Although highly effective vaccines exist for EV71, no vaccine is available for the global public health threats imposed by CVA6, which underscores the critical need for developing an effective vaccine. Here, we demonstrate the isolation of two stable CVA6 particles with excellent natural antigenicity: one empty (CVA6 procapsid) and the other infectious (CVA6 A-particle). The capsid structures of CVA6 procapsid and A-particle at near atomic (~3 Å) resolution both closely resemble those of the uncoating intermediates of other enteroviruses. The cryoEM structures of the CVA6 procapsid, A-particle, and A-particle-1D5 immune-complex we report here reveal atomic resolution details about molecular determinants in CVA6 related to virus neutralization, cell binding, and RNA release.

The top band exhibited a λ260/λ280 absorbance ratio of 0.71, and the particles in that band sedimented with a coefficient of 84S, had a capsid protein composition consistent with the presence of VP0, VP1, and VP3 in sodium dodecyl supfate–polyacrylamide gel electrophoresis (SDS–PAGE) gel electrophoresis (lane 2), and showed an absence of packaged genome as verified by negative stain electron microscopy. These characteristics are all consistent with this band being composed of purified procasids. A total of 10,749 procapsid and 7152 A-particle images were extracted and subjected to three-dimensional (3D) reconstruction, respectively, yielding final density maps at estimated resolutions of 3.3 and 3.1 Å. The density maps of the procapsid and A-particle reveal essentially identical (0.96 correlation coefficient), pseudo T = 3 icosahedral capsid structures, which explains why the two particles share similar antigenicity. The obvious difference between two density maps is the density of genomic RNA, which is present in A-particles but absent in procapsids. Atomic models of their biological protomers (VP0 + VP1 + VP3 for the procapsid and VP1 + VP2 + VP3 for the A-particle) were built manually and subsequently refined by Phenix. The structural similarity between the two atomic models was deemed quite high as judged by their superposition and confirmed by an r.m.s.d. value of 0.4 Å between the two models. Though the procapsid was shown by SDS–PAGE to contain VP0 (containing the sequences of VP2 and VP4), only the VP0 sequence corresponding to VP2 is well resolved in the density map and hence successfully modeled, indicating the one corresponding to VP4 is flexible as that in previously reported EV71 procapsid. The first 70 residues at the N-terminus of VP1 are missing in both models; The AB loop of VP2 in the A-particle contains a flexible segment of 10 a.a., but 20 a.a. in the procapsid; In VP3, one small segment (a.a.74–77) is missing in the procapsid, whereas the corresponding segment in the A-particle is intact.

> NDPIANAVESAVSALADTTISRVTAANTTASTHSLGTGRVPALQAAETGASSNASDENLVETRCVMNRNGVNEASVEHFYSRAGLVGVVEVKDSGTSLDGYTVWPIDVMGFVQQRRKLELSTYMRFDAEFTFVSNLSNSTTPGMLLQYMYVPPGAPKPDGRKSYQWQTATNPSVFAKLSDPPPQVSVPFMSPATAYQWFYDGYPTFGEHKQATNLQYGQCPNNMMGHFAIRTVSESTTGKNVHVRVYMRIKHVRAWVPRPLRSQAYMVKNYPTYSQTITNTATDRASITTTDYEGGVPASPQRTS;> MGAQVSTQKSGSHETRNVATEGSTINFTNINYYKDSYAASASRQDFAQDPAKFTRPVLDTIREVAAPLQSPSVEACGYSDRVAQLTVGNSTITTQEAANIVLSYGEWPEYCPSTDATAVDKPTRPDVSVNRFYTLSTKSWKTESTGWYWKFPDVLNDTGVFGQNAQFHYLYRSGFCMHVQCNASKFHQGALLVAAIPEFVIAASSPATKPNGRGLYPDFAHTNPGKDGQEFRDPYVLDAGIPLSQALVFPHQWINLRTNNCATIIMPYVNALPFDSALNHSNFGLVVIPISPLKYCNGATTEVPVTLTIAPLNSEFSGLRQAIKQ;> GFPTELKPGTNQFLTTDDGTSPPILPGFEPTPLIHIPGEFTSLLDLCQIETILEVNNTTGTIGVSRLLIPVRAQNNVDQLCASFQVDPGRNGPWQSTMVGQICRYYTQWSGSLKVTFMFTGSFMATGKMLIAYTPPGSAQPATREAAMLGTHIVWDFGLQSSVTLVIPWISNTHFRAVKIGGVYDYYATGIVTIWYQTNFVVPPDTPTEANIIALGAAQKNFTLKLCKDTDEIQQTAAYQ> SNAMIDAKQLNSLALAYMGDAVYEQYIRYHLLQKGKVRPNQLHRLGTSFVSAKAQA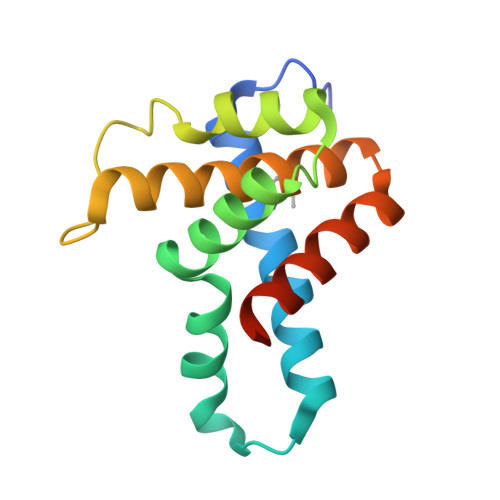KVVYHLLETAFLTEEEEAVLRRGRNANSGTVPKNTDVQTYRHSTAFEALIGYHHLLNNRERLDEIVYKAIAVLEEQEGGTSS For the levan utilisation system, the cell surface components are Bt1760 (a GH32 endo-levanase), Bt1761 (a surface glycan-binding protein; SGBP), Bt1762 (SusD) and Bt1763 (SusC)15,19,24. SusC proteins are unique among TBDTs in that they are tightly associated with a SusD substrate-binding lipoprotein15–17. Recently, we showed that SusCD complexes mediate substrate uptake via a “pedal bin” mechanism. The SusC transporter forms the barrel of the bin, while SusD sits on top of the barrel, opening and closing like a lid to facilitate substrate binding.

To visualise potential different conformational states, we used single-particle cryo-EM on detergent-solubilised apo-Bt1762-63. Strikingly, several distinct conformations of the SusC2D2 complex are present in a single dataset, and after further classification steps, three dominant states were identified. Following three-dimensional (3D) reconstruction, electron density maps were obtained at resolutions allowing rigid body placement and refinement of individual protomers. This yielded structures corresponding to the three possible combinations of open and closed dimeric transporters: OO (3.9 Å), OC (4.7 Å) and CC (4.2 Å). With the exception of a few Bt1763 loops (L6 and L7) and the Bt1762 segment following the lipid anchor that serves as a pivot around which Bt1762 moves upon lid opening, the conformational changes between the three states correspond to rigid body movements of Bt1762. Interestingly, the presence of the plug domain in the interior of the Bt1763 barrel in solution is strictly correlated with the open vs. closed state of the transporter; only open states contain a plug domain, regardless of the state of the SusC2D2 dimer. In the open, apo state of the SusCD transporter as observed via cryo-EM, the Ton box of Bt1763 (82DEVVVTG88) is visible, tucked away inside the barrel, and interacts with the body of the plug. Hinge1 and 2 change conformation substantially during lid opening and are responsible for the majority of interactions between Bt1762 and Bt1763 in the open state.

> CDDFLDRQVPQGIVTGDQIASPEYVDNLVISAYAIWATGDDINSSFSLWNYDVRSDDCYKGGSGTEDGGVFNALEISKGINTTDWNINDIWKRLYQCITRANTALQSLDQMDEKTYPLKNQRIAEMRFLRGHAHFMLKQLFKKIVIVNDENMEPDAYNELSNTTYTNDEQWQKIADDFQFAYDNLPEVQIEKGRPAQAAAAAYLAKTYLYKAYRQDGADNALTGINEEDLKQVVKYTDPLIMAKGGYGLETDYSMNFLPQYENGAESVWAIQYSINDGTYNGNLNWGMGLTTPQILGCCDFHKPSQNLVNAFKTDSQGKPLFSTYDNENYEVATDNVDPRLFHTVGMPGFPYKYNEGYIIQKNDDWSRSKGLYGYYVSLKENVDPDCDCLKKGSYWASSLNHIVIRYADVLLMRAEALIQLNDGRITDAISLINEVRSRAAGSTMLIFNYKEDYGVNFKVTPYDLKAYAQDEAMKMLKWERRVEFGMESSRFFDLVRWGEAKDVINAYYVTEASRCSIYKNAGFTENKNEYLPVPFEQISASNGNYTQNFGWAAAAHHHHHH;> VVVTGYTTQRKADLTGAVSVVKVDEIQKQGENNPVKALQGRVPGMNITADGNPSGSATVRIRGIGTLNNNDPLYIIDGVPTKAGMHELNGNDIESIQVLKDAASASIYGSRAANGVIIITTKQGKKGQIKINFDASVSASMYQSKMNVLNTEQYGRAMWQAYVNDGENPNGNALGYAYNWGYNADGNPVLYGMTLSKYLDSKNTMPVADTDWFDEITRTGVIQQYNLSVSNGSEKGSSFFSLGYYKNLGVIKDTDFDRFSARMNSDYKLIDDILTIGQHFTLNRTSEVQAPGGIIETALDIPSAIPVYASDGSWGGPVGGWPDRRNPRAVLEYNKDNRYTYWRMFGDAYVNLTPFKGFNLRSTFGLDYANKQARYFTYPYQEGTQTNNGKSAVEAKQEHWTKWMWNAIATYQLEVGKHRGDVMIGMELNREDDSHFSGYKEDFSILTPDYMWPDAGSGTAQAYGAGEGYSLVSFFGKMNYSYADRYLLSLTLRRDGSSRFGKNHRYATFPSVSLGWRITQENFMKELTWLDDLKLRASWGQTGNQEISNLARYTIYAPNYGTTDSFGGQSYGTAYDITGSNGGGVLPSGFKRNQIGNDNIKWETTTQTNVGIDFSLFKQSLYGSLEYYYKKATDILTEMAGVGVLGEGGSRWINSGAMKNQGFEFNLGYRNKTAFGLTYDLNGNISTYRNEILELPETVAANGKFGGNGVKSVVGHTYGAQVGYIADGIFKSQDEVDNHATQEGAAVGRIRYRDIDHNGVIDERDQNWIYDPTPSFSYGLNIYLEYKNFDLTMFWQGVQGVDIISDVKKKSDFWSASNVGFLNKGTRLLNAWSPTNPNSDIPALTRSDTNNEQRVSTYFVENGSFLKLRNIQLGYTVPAVISKKMRMDRLRFYCSAQNLLTIKSKNFTGEDPENPNFSYPIPVNITFGLNIGF Staphylococcus aureus (SA) leukocidin ED (LukED) belongs to a family of bicomponent pore forming toxins that play important roles in SA immune evasion and nutrient acquisition. LukED targets specific G protein-coupled chemokine receptors to lyse human erythrocytes (red blood cells) and leukocytes (white blood cells). Each leukotoxin is made up of two subunits of approximately 30 kDa: a host cell targeting S-component (HlgA, HlgC, LukE, lukS-PV, and LukA/G), and a polymerization F- component (HlgB, LukD, lukF-PV, and LukB/H), which can bind the plasma membrane through highly conserved phosphocholine binding sites. Each toxin is composed of two domains: a central β sandwich called the CAP domain and involved in inter-protomer interactions, and a RIM domain which contains several divergent loops driving host cell specificity.

Unexpectedly, we found two bound copies of the peptide, which may be due to the potentially very high peptide concentration used during crystal soaking experiments. Residues 34–43, and residues 39–46 are visible for the 1st and 2nd peptide, respectively. The first peptide interacts with site 1 through its sTyr41 residue in a manner similar to the pCS molecule. The preceding residues 36FPDGD40 close the back of the binding pocket, decreasing the solvent exposed surface area of sTyr41, and provide additional stability through multiple intermolecular interactions. Asp38 forms a salt bridge with LukE Arg290, and Gly39 carbonyl oxygen is hydrogen bonded to Arg101 from site 2. The 2nd peptide sTyr41 residue interacts with site 2, in a way that is also similar to pCS, although Arg101 sidechain adopts a different conformation and an additional salt bridge is formed between the sulfate and Lys283. Other stabilizing interactions include several backbone-backbone hydrogen bonds between Asp40-Lys92, Gly42-Asp90, and Leu45-Phe88, and hydrophobic interactions between Leu45 and Phe88, Ala219 and Arg220 of LukE. Although the conformation of both peptides is stabilized by multiple interactions with LukE, it should be noted that the 2nd peptide chain runs with its C-terminus going away from the putative location of the membrane. In addition, the occupancy is relatively low (except for the sulfotyrosines) and the conformation of the peptides is likely influenced by crystal packing and the associated steric constraints.

> MSVGLIAPLASPIQESRANTNIENIGDGAEVIKRTEDVSSKKWGVTQNVQFDFVKDKKYNKDALIVKMQGFINSRTSFSDVKGSGYELTKRMIWPFQYNIGLTTKDPNVSLINYLPKNKIETTDVGQTLGYNIGGNFQSAPSIGGNGSFNYSKTISYTQKSYVSEVDKQNSKSVKWGVKANEFVTPDGKKSAHDRYLFVQSPNGPTGSAREYFAPDNQLPPLVQSGFNPSFITTLSHEKGSSDTSEFEISYGRNLDITYATLFPRTGIYAERKHNAFVNRNFVVRYEVNWKTHEIKVKGHNKHHHHHH;>XDSFPDGDYGANLE[2x]>MDFTKPETVLNLQNIRDELVRMEDSIIFKFIERSHFATCPSVYEANHPGLEIPNFKGSFLDWALSNLEIAHSRIRRFESPDETPFFPDKIQKSFLPSINYPQILAPYAPEVNYNDKIKKVYIEKIIPLISKRDGDD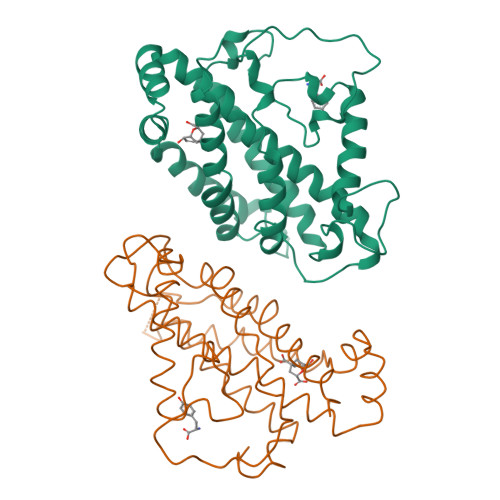KNNFGSVATRDIECLQSLSRRIHFGKFVAEAKFQSDIPLYTKLIKSKDVEGIMKNITNSAVEEKILERLTKKAEVYGVDPTNESGERRITPEYLVKIYKEIVIPITKEVEVEYLLRRLEE[2x]>[4x]MANTAFVSS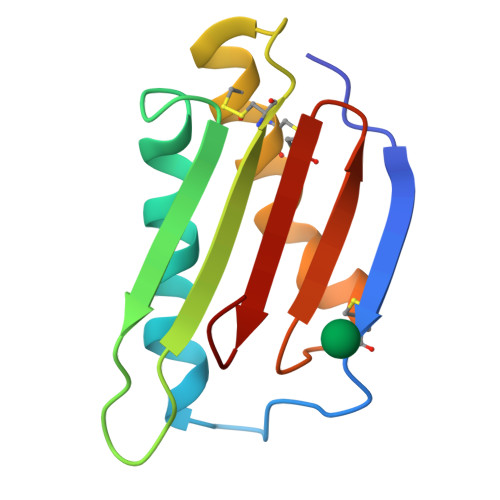ACNTQKIPSGSPFNRNLRAMLADLRQNTAFSGYDYKTSRAGSGGAPTAYGRATCKQSISQSDCTACLSNLVNRIFSICNNAIGARVQLVDCFIQYEQRSF>[2x]MRKAAGKYGNTLEFGHLVGGEEVLEGPLLERRNPSDREDVVARFPEADKDLVRKAALKAREAFAEWSRTPAPIRGQVLFNLVKILEREKPTLTRLMVREVGKTPKEAAGDVQEAIDTALFFASEGRRLYGQTVPSEMRDKELFTFRRPLGVVGIITAGNFPIAVPSWKLIPAVLTGNTVVWKPSEDAPTLSFVFAKLFEEAGLPPGVLNVVFGGGKGSTGQWMVELMDEGLFQKFAFTGSTQVGRWIGEVAGRNLIRPTLELGGKNPLVVMRDADLDLAVEGAWWSAFATGGQRCTSAGNILVDAPIYEEFKRRFLERVEATLVGNPLLHPEVTYGPFINERFFARWQEHYRVGEAEGARLLFGRGRITRENPYPRFLGDPEAGLYGWPTVWEVRPGTRLFTEEVFGPTINLVKVDGIEEAIAVANSTPYGLSSAIYTNHRHWAYLFKVGIRAGMTSINNATVGAEAH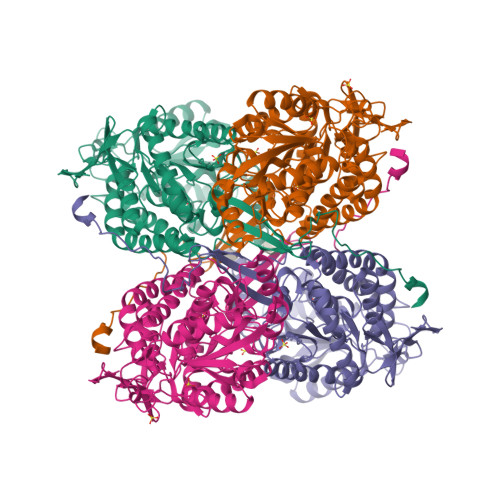LPFGGVKASGNGGRESGIWVLEEYTYWHAVNEEYSGRLQLAQMDTGYVSPKAPTPWGEVLGL>MGSSHHHHHHSSGENLYFQGSQIHVDTMKVINDPIHGHIELHPLLVRIIDTPQFQRLRYIKQLGGGYYVFPGASHNRFEHSLGVGYLAGCLVHALGEKQPELQISERDVLCVQIAGLCHDLGHGPFSHMFDGRFIPLARPEVKWTHEQGSVMMFEHLINSNGIKPVMEQYGLIPEEDIYFIKEQIVGPLESPVEDSLWPYKGRPENKSFLYEIVSNKRNGIDVDKWDYFARDCHHLGIQNNFDYKRFIKFARVCEVDNELRICARDKEVGNLYDMFHTRNSLHRRAYQHKVGNIIDTMITDAFLKADDYIEITGAGGKKYRISTAIDDMEAYTKLTDNIFLEILYSTDPKL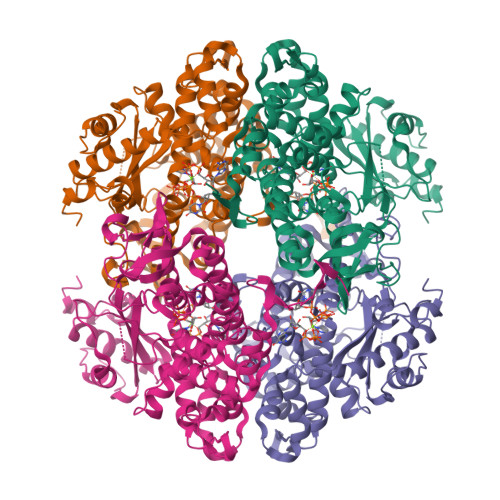KDAREILKQIEYRNLFKYVGETQPTGQIKIKREDYESLPKEVASAKPKVLLDVKLKAEDFIVDVINMDYGMQEKNPIDHVSFYCKTAPNRAIRITKNQVSQLLPEKFAEQLIRVYCKKVDRKSLYAARQYFVQWCADRNFTKPQDGDVIAPLITPQKKEWNDSTSVQNPTRLREASKSRVQLFKDDPM[2x]>[2x]MGSSHHHHHHGSMYGVYRAMKLPIYLDYSATTPVDPRVAEKMMQFMTMDGTFGNPASRSHRFGWQAEEAVDIARNQIADLVGADPREIVFTSGATESDNLAIKGAANFYQKKGKHIITSKTEHKAVLDTCRQLEREGFEVTYLAPQRNGIIDLKELEAAMRDDTILVSIMHVNNEIGVVQDIAAIGEMCRARGIIYHVDATQSVGKLPIDLSQLKVDLMSFSGHKIYGPKGIGALYVRRKPRVRIEAQMHGGGHERGMRSGTLPVHQIVGMGEAYRIAKEEMATEMERLRGLRNRLWNGIKDIEEVYLNGDLEHGAPNILNVSFNYVEGESLIMALKDLAVSSGSACTSASLEPSYVLRALGLNDELAHSSIRFSLGRFTTEEEIDYTIELVRKSIGRLRDLSPLWEMYKQG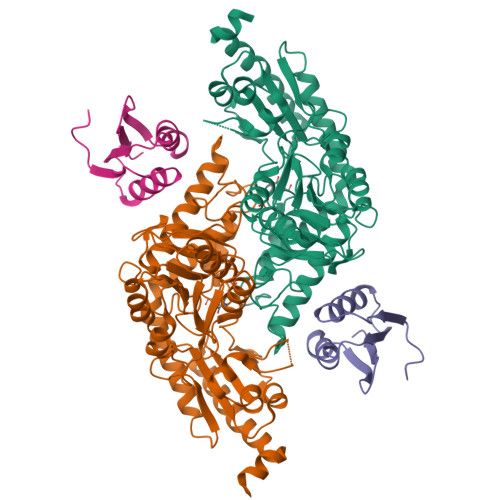VDLNSIEWAHH;>[2x]GSTDLFSSPDHTLDALGLRCPEPVMMVRKTVRNMQPGETLLIIADDPATTRDIPGFCTFMEHELVAKETDGLPYRYLIRKGG> MEELEQGLLMQPWAWLQLAENSLLAKVFITKQGYALLVSDLQQVWHEQVDTSVV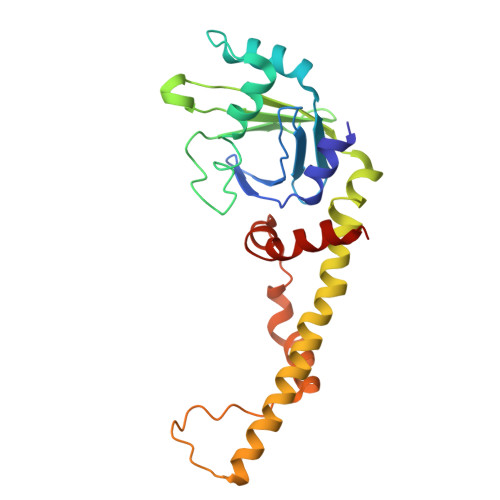SQRAKELNKRLTAPPAAFLCHLDNLLRPLLKDAAHPSEATFSCDCVADALILRVRSELSGLPFYWNFHCMLASPSLVSQHLIRPLMGMSLALQCQVRELATLLHMKDLEIQDYQESGATLIRDRLKTEPFEENSFLEQFMIEKLPEACSIGDGKPFVMNLQDLYMAVTTQHHHHHH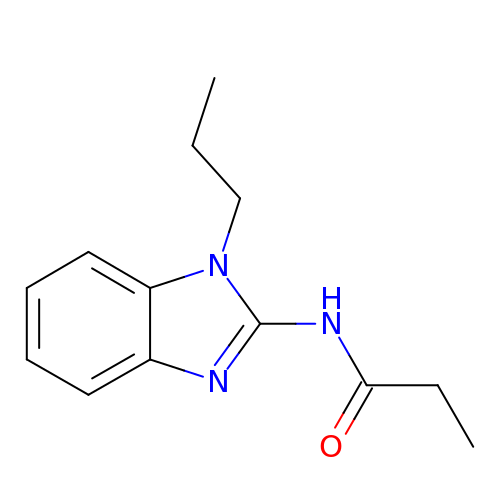~{N}-(1-propylbenzimidazol-2-yl)propanamide | C13 H17 N3 O | KFQGOQCGYCFOQG-UHFFFAOYSA-N> SRAN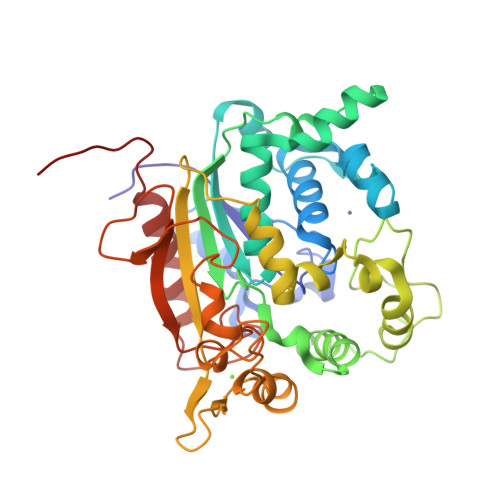DAPIVLLHGFTGWGREEMFGFKYWGGVRGDIEQWLNDNGYRTYTLAVGPLSSNWDRACEAYAQLVGGTVDYGAAHAAKHGHARFGRTYPGLLPELKRGGRIHIIAHSQGGQTARMLVSLLENGSQEEREYAKAHNVSLSPLFEGGHHFVLSVTTIATPHDGTTLVNMVDFTDRFFDFQKAVLKAAAVASNVPYTSQVYDFKLDQWGLRRQPGESFDQYFERLKRSPVWTSTDTARYDLSVPGAEKLNQWVKASPNTYYLSFATERTYRGALTGNYYPELGMNAFSAVVCAPFLGSYRNATLGIDDRWLENDGIVNAFSMNGPKRGSTDRIVPYDGTIKKGVWNDMGTYNVDHLEVIGVDPNPLFDIRAFYLRLAEQLASLQPHHHHHH>[7x]STSAGPTVPDRDNDGIPDSLEVEGYTVDVKNKRTFLSPWISNIHEKKGLTKYKSSPEKWSTASDPYSDFEKVTGRIDKNVSPEARHPLVAAYPIVHVDMENIILSKNEDQSTQNTDSQTRTISKNTSTSRTHTSEVHGNAEVHASFFDIGGSVSAGFSNSNSSTVAIDHSLSLAGERTWAETMGLNTADTARLNANIRYVNTGTAPIYNVLPTTSLVLGKNQTLATIKAKENQLSQILAPNNYYPSKNLAPIALNAQDDFSSTPITMNYNQFLELEKTKQLRLDTDQVYGNIATYNFENGRVRVDTGSNWSEVLPQIQETTARIIFNGKDLNLVERRIAAVNPSDPLETTKPDMTLKEALKIAFGFNEPNGNLQYQGKDITEFDFNFDQQTSQNIKNQLAELNATNIYTVLDKIKLNAKMNILIRDKRFHYDRNNIAVGADESVVKEAHREVINSSTEGLLLNIDKDIRKILSGYIVEIEDTEGLKEVINDRYDMLNISSLRQDGKTFIDFKKYNDKLPLYISNPNYKVNVYAVTKENTIINPSENGDTSTNGIKKILIFSKKGYEIG;> MNIKKEFIKVISMSCLVTAITLSGPVFIPLVQGAGGHGDVGMHVKEKEKNKDENKRKDEERNKTQEEHLKEIMKHIVKIEVKGEEAVKKEAAEKLLEKVPSDVLEMYKAIGGKIYIVDGDITKHISLEALSEDKKKIKDIYGKDALLHEHYVYAKEGYEPVLVIQSSEDYVENTEKALNVYYEIGKILSRDILSKINQPYQKFLDVLNTIKNASDSDGQDL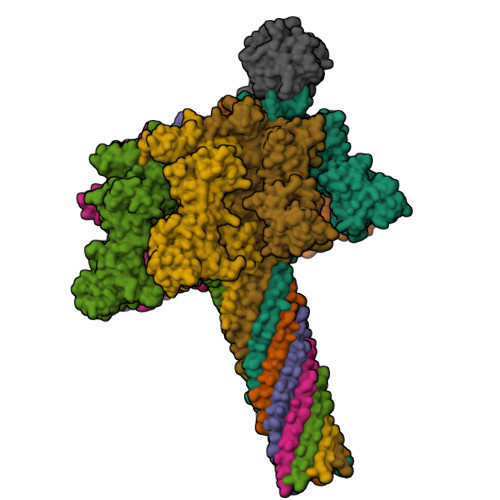LFTNQLKEHPTDFSVEFLEQNSNEVQEVFAKAFAYYIEPQHRDVLQLYAPEAFNYMDKFNEQEINLSLEELKDQRMLARYEKWEKIKQHYQHWSDSLSEEGRGLLKKLQIPIEPKKDDIIHSLSQEEKELLKRIQIDSSDFLSTEEKEFLKKLQIDIRDSLSEEEKELLNRIQVDSSNPLSEKEKEFLKKLKLDIQPYDINQRLQDTGGLIDSPSINLDVRKQYKRDIQNIDALLHQSIGSTLYNKIYLYENMNINNLTATLGADLVDSTDNTKINRGIFNEFKKNFKYSISSNYMIVDINERPALDNERLKWRIQLSPDTRAGYLENGKLILQRNIGLEIKDVQIIKQSEKEYIRIDAKVVPKSKIDTKIQEAQLNINQEWNKALGLPKYTKLITFNVHNRYASNIVESAYLILNEWKNNIQSDLIKKVTNYLVDGNGRFVFTDITLPNIAEQYTHQDEIYEQVHSKGLYVPESRSILLHGPSKGVELRNDSEGFIHEFGHAVDDYAGYLLDKNQSDLVTNSKKFIDIFKEEGSNLTSYGRTNEAEFFAEAFRLMHSTDHAERLKVQKNAPKTFQFINDQIKFIINS>GSGMMRYLHKIELELNRLTSRYPFFKKIAFDAEIIKLVDDLNVDENVKCAIVAIDTSMRMQDFINEDNKDSFVLSTDVLSALFYKYLSQPFYQHDFLVLTDCVSRINELKSIRATITDEIALHNINKQIHYMFIQPYMNNEKVVSYE[2x];>MIALSYKAFLNPYIIEVEKRLYECIQSDSETINKAAHHILSSGGKRVRPMFVLLSGFLNDTQKDDLIRTAVSLELVHMASLVHDDYIDNSDMRRGNTSVHIAFDKDTAIRTGHFLLARALQNIA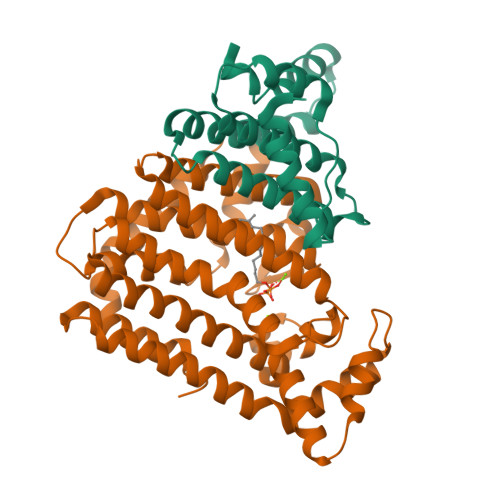TINNSKFHQIFSKTILEVCFGEFDQMADRFNYPVSFTAYLRRINRKTAILIEASCHLGALSSQLDEQSTYHIKQFGHCIGMSYQIIDDILDYTSDEATLGKPVGSDIRNGHITYPLMAAIANLKEQDDDKLEAVVKHLTSTSDDEVYQYIVSQVKQYGIEPAELLSRKYGDKAKYHLSQLQDSNIKDYLEEIHEKMLKRVY[2x]> GGMGNNSRASNPVPLEDQIGALLGEHPRQIVPLHAGRRAQVLRCHFQDGHSVIVKSFTEVAETTRGEWDALRFLAAHVPAIAPRPLARSKDRRLVAMEDLRGETLARLLERESEAGARRPLVRIADALGHLHGAQAPRVDGLPRALRDEYRKQADECVALRGKVRALLGRAGVEPTPGFDGAWLELVERMGSPGPFLTFTHGDLAPSNVLLTDDGPRLLDFEYTGARSALYDVMFWEAVVPFPRSLARPMTQAYRRALASHLPAARDDARFRRELLTLKTHRFFWWLTFRLDEALAGGDAHWVPGWRLRPAYLFYLQNYVSTARRLGARGPLLKTAQALSSRLRRGWKERA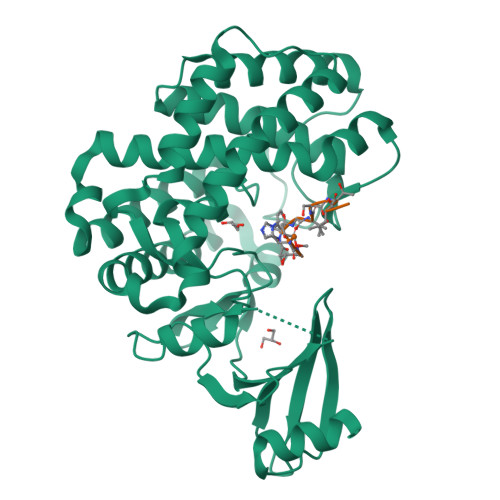GYPDHFLGKLKPPGP>[3x]GHMSPFTGSAAPTPEWRHLRVEITDGVATVTLARPDKLNALTFEAYADLRDLLAELSRRRAVRALVLAGEGRGFCSGGDVDEIIGATLSMDTARLLDFNRMTG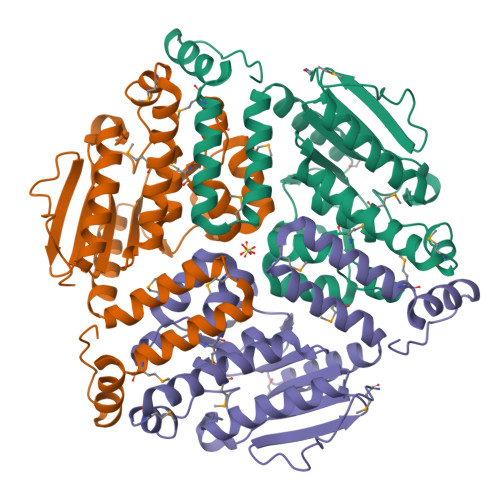QVVRAVRECPFPVIAALHGVAAGAGAVLALAADFRVADPSTRFAFLFTRVGLSGGDMGAAYLLPRVVGLGHATRLLMLGDTVRAPEAERIGLISELTEEGRADEAARTLARRLADGPALAHAQTKALLTAELDMPLAAAVELDASTQALLMTGEDYAEFHAAFTEKRPPKWQGRGS> GGSHMKSYEIALIGNPNVGKSTIFNALTGENVYIGNWPGVTVEKKEGEFEYNGEKFKVVDLPGVYSLTANSIDEIIARDYIINEKPDLVVNIVDATALERNLYLTLQLMEMGANLLLALNKMDLAKSLGIEIDVDKLEKILGVKVVPLSAAKKMGIEELKKAISIAVKDKKTAEIKYPNFEPYIKKI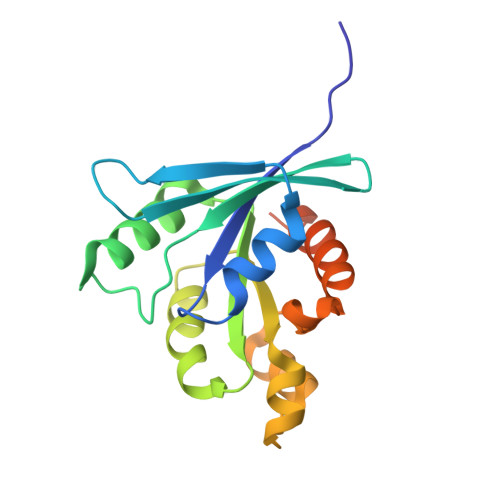T>[2x]MPEIITPIITPFTKDNRIDKEKLKIHAENLIRKGIDKLFVNGTTGLGPSLSPEEKLENLKAVYDVTNKIIFQVGGLNLDDAIRLAKLSKDFDIVGIASYAPYFYPRMSEKHLVKYFKTLCEVSPHPVYLFNYPTATGKDIDAKVAKEIGCFTGVKDTIENIIHTLDYKRLNPNMLVYSGSDMLIATVASTGLDGNVAF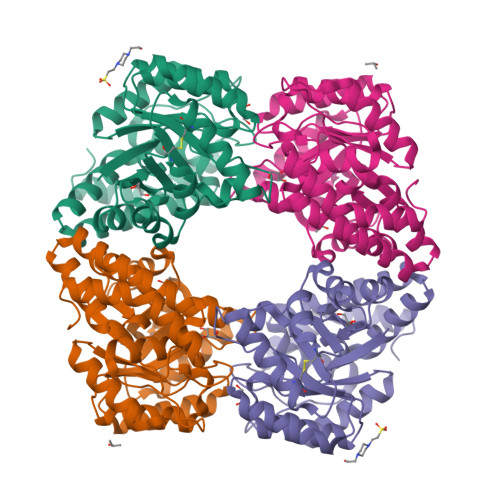GSNYLPEVTVTIKKLAMERKIDEALKLQFLHDEVIEASRIFGSLSSNYVLTKYFQGYDLGYPRPPIFPLDDEEERQLIKKVEGIRAKLVELKILKE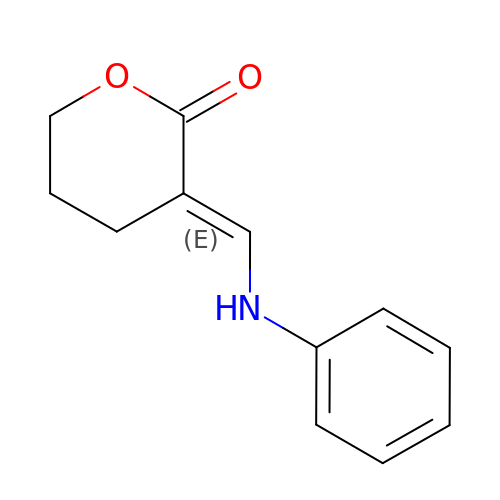(3E)-3-[(phenylamino)methylidene]oxan-2-one | C12 H13 N O2 | OFOTXGOGHOCRQE-MDZDMXLPSA-N3-(5-{[4-(AMINOMETHYL)PIPERIDIN-1-YL]METHYL}-1H-INDOL-2-YL)-1H-INDAZOLE-6-CARBONITRILE | 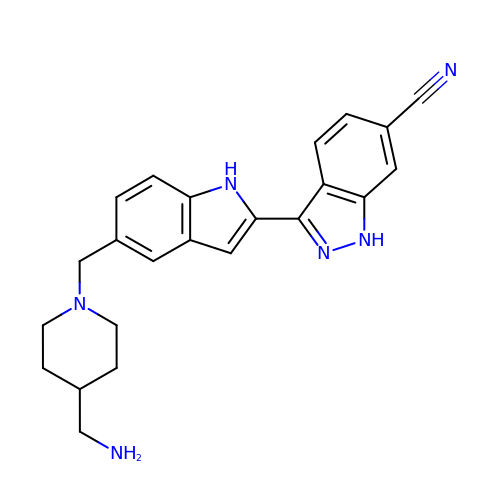C23 H24 N6 | WBKUBPBCFYCSRT-UHFFFAOYSA-N>[11x]MEKFRAVLDLHVKHHSALGYGLVTLLTAGGERIFSAVAFQCPCSAAWNLPYGLVFLLVPALALFLLGYVLSARTWRLLTGCCSSARASCGSALRGSLVCTQISAAAALAPLTWVAVALLGGAFYECAATGSAAFAQRLCLGRNRSCAAELPLVPCNQAKASDVQDLLKDLKAQSQVLGWILIAVVIIILLIFTSVTRCLSPVSFLQLKFWKIYLEQEQQILKSKATEHATELAKENIKCFFEGSHPKE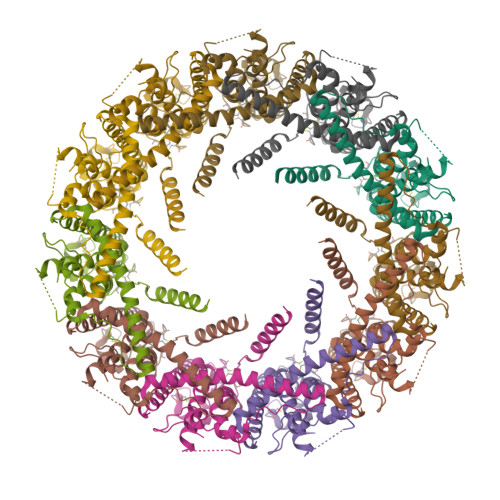YNTPSMKEWQQISSLYTFNPKGQYYSMLHKYVNRKEKTHSIRSTEGDTVIPVLGFVDSSGINSTPEL>MHHHHHHGSEVEIKFKIKLEDFLHTLNTFNPEFVRYEEQEDVYFEVPRPKLLRIRGVHNLKKYYLTFKEILDENNEEFYEVEFEIGDFEKAVEVFKRLGFKIQATIKKKRWVYKLNGVTLEVNRVEGIGDFVDIEVISDSPEEAKEKIWEVAKMLGLKEEDVEPRLYLELINELS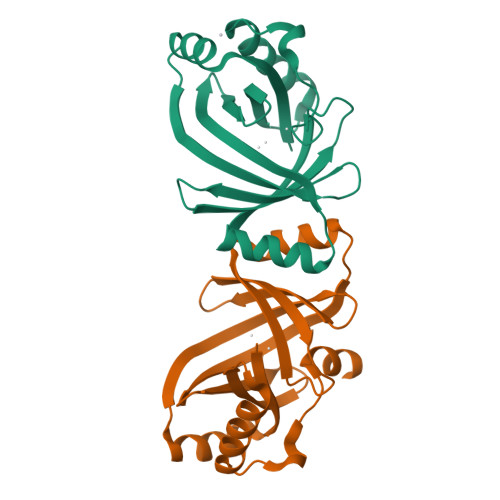GRSS[2x]6-(benzyloxy)-9H-purin-2-amine 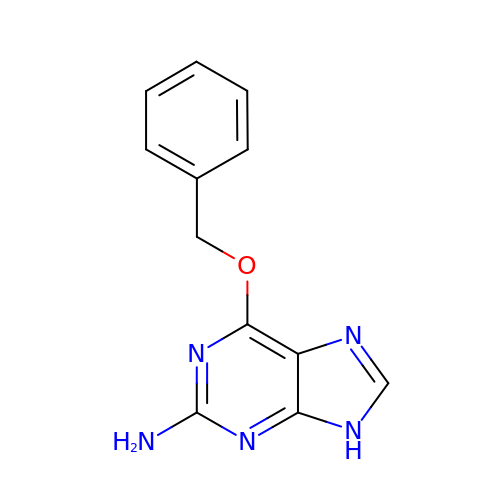| C12 H11 N5 O | KRWMERLEINMZFT-UHFFFAOYSA-N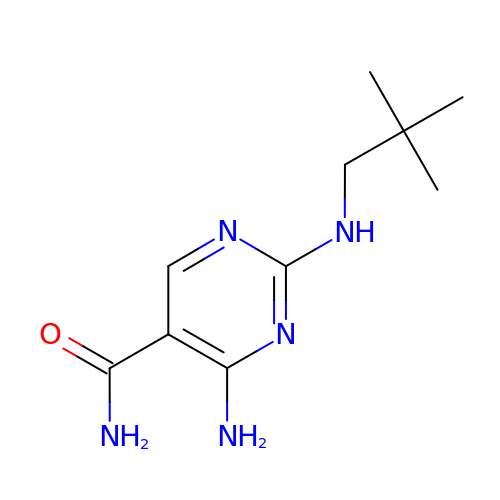4-amino-2-[(2,2-dimethylpropyl)amino]pyrimidine-5-carboxamide | C10 H17 N5 O | PYEPYUBHFUICHO-UHFFFAOYSA-N>MAKHATPKLDQLESGPWPSFVSDIKQEAAYRAANPKGLDYQVPVDCPEDLLGVLELSYDEGETHWKHGGIVGVFGYGGGVIGRYCDQPEKFPGVAHFHTVRVAQPSGKYYSADYLRQLCDIWDLRGSGLTNMHGSTGDIVLLGTQTPQLEEIFFELTHNLNTDLGGSGSNLRTPESCLGKSRCEFACYDSQAACYELTMEYQDELHRPAFPYKFKFKFDACPNGCVASIARSDFSVIGTWKDDIKIDAEAVKAYVAGEFKPNAGAHSGRDWGKFDIEAEVVNRCPSKCMKWDGSKLSIDNKECVRCMHCINTMPRALHIGDERGASILCGAKAPILDGAQMGSLLVPFVAAEEPFDEIKEVVEKIWDWWMEEGKNRERLGETMKRLSFQKLLEVTEIAPVPQHVKEPRTNPYIFFKEEEVPGGWDRDITEYRKRHLR[2x];>MAFISSGYNPEKPMANRITDIGPRKFDEFFPPVIAKNFGSWLYHEILEPGVLMHVAESGDKVYTVRVGAARLMSITHIREMCDIADKYCGGHLRFTTRNNVEFMVADEASLKALKEDLASRKFDGGSLKFPIGGTGAGVSNIVHTQGWVHCHTPATDASGPVKAIMDEVFEDFQSMRLPAPVRISLACCINMCGAVHCSDIGVVGIHRKPPMIDHEWTDQLCEIPLAVASCPTAAVRPTKLEIGDKKVNTIAIKNERCMYCGNCYTMCP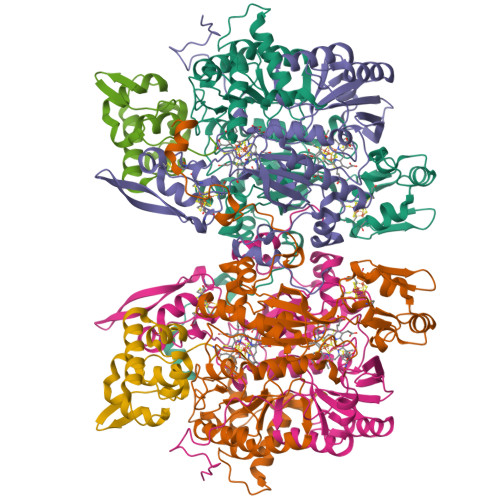ALPISDGEGDGVVIMVGGKVSNRISMPKFSKVVVAYIPNEPPRWPSLTKTIKHIIEVYSANAYKYERLGEWAERIGWERFFSLTGLEFSHHLIDDFRDPAYYTWRQSTQFKF[2x];>MAEVTYKGKSFEVDEDGFLLRFDDWCPEWVEYVKESEGISDISPDHQKIIDFLQDYYKKNGIAPMVRILSKNTGFKLKEVYELFPSGPGKGACKMAGLPKPTGCV[2x]> CAGCAGCCTGAATA;> GGCTGC;> GCGAGTATTCA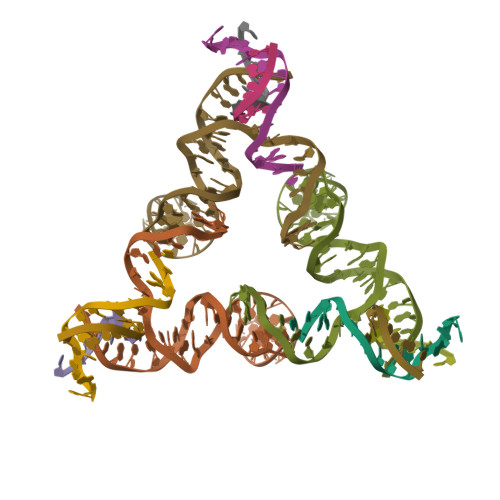CCGGCTCCGCGGTTTTCCGCGGCTCGCAGCCGGACAGCG;> TGCGCTGT>GPGSMAAATFHWDDPLLLDQQLADDERMVRDAAHAYAQGKLAPRVTEAFRHETTDAAIFREMGEIGLLGPTIPEQYGGPGLDYVSYGLIAREVERVDSGYRSMMSVQSSLVMVPIFEFGSDAQKEKYLPKLATGEWIGCFGL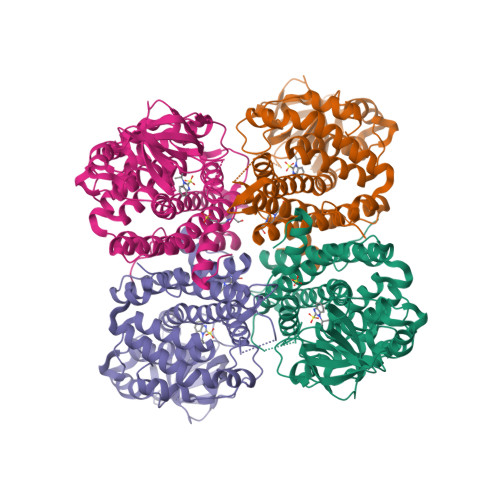TEPNHGSDPGSMVTRARKVPGGYSLSGSKMWITNSPIADVFVVWAKLDEDGRDEIRGFILEKGCKGLSAPAIHGKVGLRASITGEIVLDEAFVPEENILPHVKGLRGPFTCLNSARYGIAWGALGAAESCWHIARQYVLDRKQFGRPLAANQLIQKKLADMQTEITLGLQGVLRLGRMKDEGTAAVEITSIMKRNSCGKALDIARLARDMLGGNGISDEFGVARHLVNLEVVNTYEGTHDIHALILGRAQTGIQAFF[4x]>[4x]DDYLDRLPKSKKGLQGLLQDIEKRILHYKQLFFKEQNEIANGKRSMVPDNSIPICSDVTKLNFQALIDAQMRHAGKMFDVIMMDPPWQLSSSQPSRGVAIAYDSLSDEKIQNMPIQSLQQDGFIFVWAINAKYRVTIKMIENWGYKLVDEITWVKK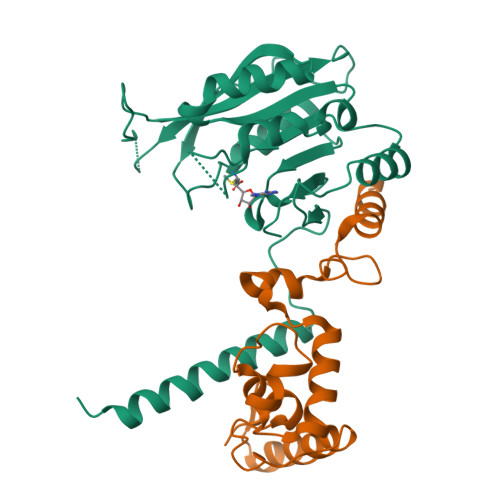TVNGKIAKGHGFYLQHAKESCLIGVKGDVDNGRFKKNIASDVIFSERRGQSQKPEEIYQYINQLCPNGNYLEIFARRNNLHDNWVSIGNEL;>MSTISREEYAKKMRLALSDNHICKPDGTVNHQYFLVKKGQYWGEEKIQYLIEQLEKIGVGNWKQMQKGLLEQTSEIELELRTCLLFKTTDIQPYMDKKFTKIEIEQIAQQNIEKAQQLSKLKYGVFVV[4x]>LPSPTPNLEIKYTKIFINNEWQNSESGRVFPVYNPATGEQVCEVQEADKADIDKAVQAARLAFSLGSVWRRMDASERGRLLDKLADLVERDRAVLATMESLNGGKPFLQAFYVDLQGVIKTFRYYAGWADKIHGMTIPVDGDYFTFTRHEPIGVCGQIIPWNFPLLMFAWKIAPALCCGNTVVIKPAEQTPLSALYMGALIKEAGFPPGVINILPGYGPTAGAAIASHIGIDKIAFTGSTEVGKLIQEAAGRSNLKRVTLELGGKSPNIIFADADLDYAVEQAHQGVFFNQGQCCTAGSRIFVEESIYEEFVRRSVERAKRRVVGSPFDPTTEQGPQIDKKQYNKILELIQSGVAEGAKLECGGKGLGRKGFFIEPTVFSNVTDDMRIAKEEIFGPVQEILRFKTMDEVIERANNSDFGLVAAVFTN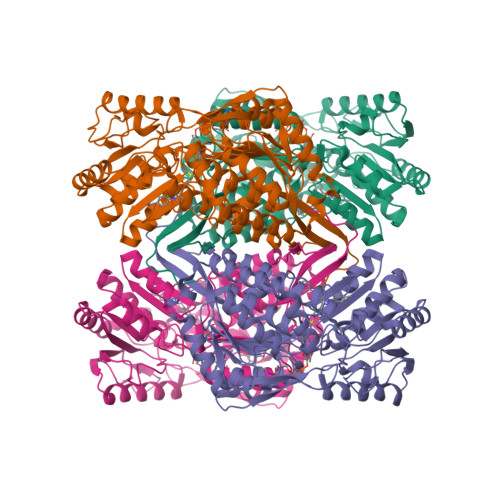DINKALTVSSAMQAGTVWINCYNALNAQSPFGGFKMSGNGREMGEFGLREYSEVKTVTVKIPQKNS[4x]> GSMSRSKRDNNFYSVEIGDSTFTVLKRYQNLKPIGSGAQGIVCAAYDAILERNVAIKKLSRPFQNQTHAKRAYRELVLMKCVNHKNIIGLLNV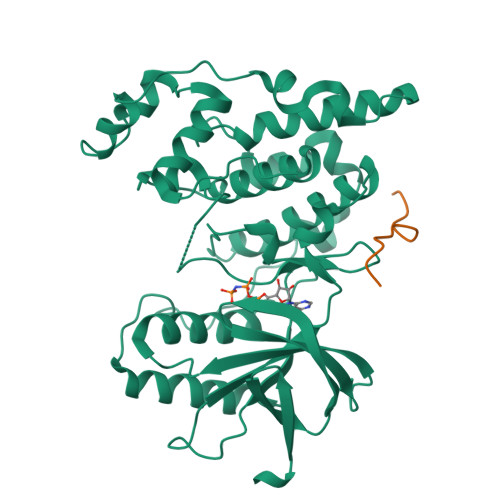FTPQKSLEEFQDVYIVMELMDANLCQVIQMELDHERMSYLLYQMLCGIKHLHSAGIIHRDLKPSNIVVKSDCTLKILDFGLARTAGTSFMMVPFVVTRYYRAPEVILGMGYKENVDIWSVGCIMGEMIKGGVLFPGTDHIDQWNKVIEQLGTPCPEFMKKLQPTVRTYVENRPKYAGYSFEKLFPDVLFPADSEHNKLKASQARDLLSKMLVIDASKRISVDEALQHPYINVWYDPSEAEAPPPKIPDKQLDEREHTIEEWKELIYKEVMDLEERTKNGVIRGQPSPLAQVQQ;> LERPSRDHLYLPLE>ADFKFEPMRSLIYVDCVSEDYRPKLQRWIYKVHIPDSISQFEPYVTKYAFY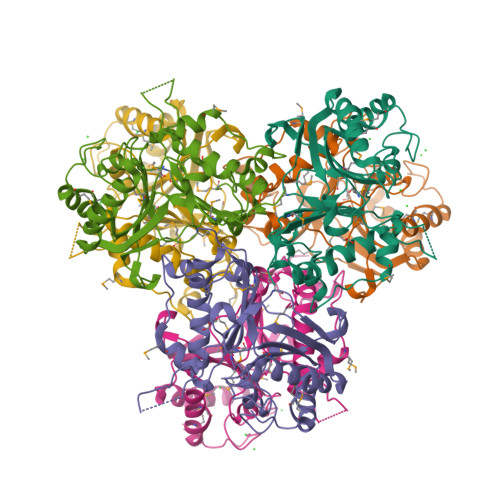PSFPIPPQGDRFGYARMQLTEHHWLVSDLDPRLEIKAIAETFPMDVLVWQGQIPAAAHTDAQIDSDGDAGNAARKSNNAEGNPFIFAFLPMWWEKDLKGKGRTIEDGANYRFNMTIGFPEGVDKAEGEKWLFEKVVPILQAAPECTRVLASAVKKDINGCVMDWVLEIWFENQSGWYKVMVDDMKALEKPSWAQQDAFPFLKPYHNVCSAAVADYTPSNNLANYRGYITMR[6x]> ADLTSHHHHHHVEPARITLTYKEGAPITIMDNGNIDTELLVGTLTLGGYKTGTTS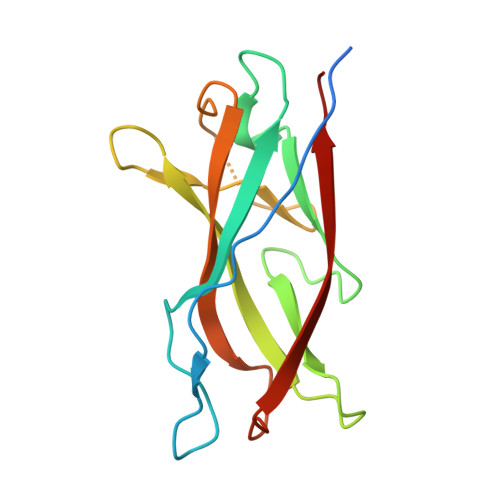TSVNFTDAAGDPMYLTFTSQDGNNHQFTTKVIGKDSRDFDISPKVNGENLVGDDVVLATGSQDFFVRSIGSKGGKLAAGKYTDAVTVTVSNQ>RSEKRDLYTQIDRLTDQRDALREKLSAADNFDIQVGSRIVHDALVGKSVVIFRTPDAHDDDIAAVSKIVGQAGGAVTATVSLTQEFVEANSAEKLRSVVNSSILPAGSQLSTKLVDQGSQAGDLLGIALLSNADPAAPTVEQAQRDTVLAALRETGFITYQPRDRIGTANATVVVTGGALSTDAGNQGVSVARFAAALAPRGSGTLLAGRDGSANRPAAVAVTRADADMAAEISTVDDIDAEPGRITVILALHDLINGGHVGHYGTGHGAMSVTVSQ[3x]

D,L-endopeptidase RipA is the major PG hydrolase required for daughter cell separation in Mycobacterium tuberculosis ( Mtb ), as RipA defects severely hinder cell division and increase antibiotic vulnerability. Despite extensive studies, the mechanisms governing Mtb RipA regulation remain controversial and poorly understood. Here, we report an integrative structural and functional analysis of the SteAB system, a regulatory complex that has been shown to modulate cell separation in the model organism Corynebacterium glutamicum ( Cglu ) and is conserved across Mycobacteriales .

Although Mtb SteB was previously proposed to act as a mycobacterial outer membrane copper transporter, the crystal structures of the homodimeric protein, alone and in complex with the RipA coiled-coil (CC) domain, rule out this hypothesis. Instead, the high-affinity SteB-RipA interaction, together with computational and biophysical data, strongly supports the role of SteB as a direct RipA activator that releases enzyme autoinhibition upon complex formation.> GARVTNKKIVSSLQTTVEADGQSSTAEKSAEVTENKDGVNVVDTIHYKGLIPKQKYEVVGILYEVKDGKLVDPNKPITISNGTGEYTVSDSGEGE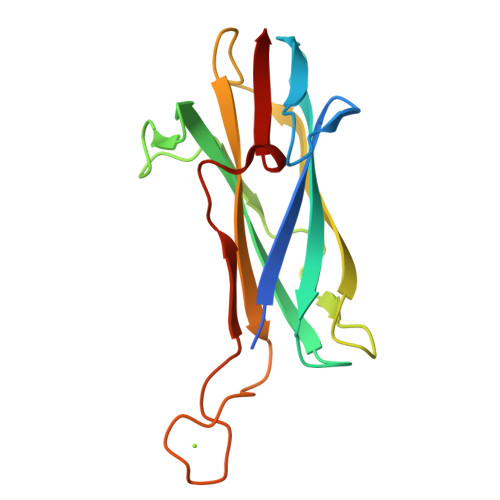WKLNFGKIDGVEARKSYVVYEEVTSVENLVDTDNDGNPDKKHEVEHKDPKDKSQTFVVKP>MVTIESDKLRQHDEQLMTKAEQFIIASYRELGKSEQEIKRRVNEIRWEVEQTGTYRHTYEELSYGAKMAWRHSNRCIGRLFWQSLHVIDAREAVTEEEVFSYLFHHIEVATNGGKIRPTITIFRPNGEVRIWNHQLIRYAGYETEEGIIGDSSSLTFTRACEQLGWKGEKTPFDVLPLVIQVGGQKPVWTPIPKELVLEVPIEHPEFPWFRDLQLKWYAVPIISDMCLEIGGIRYMAAPFNGWYMGTEIGARNFADDYRYNMLPKVASCMGLDTNSNASLWKDKA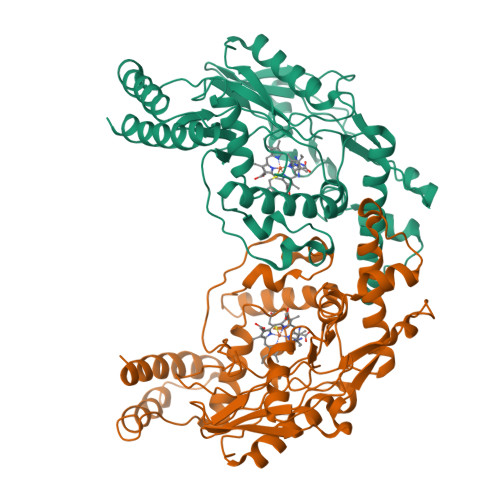LVELNIAVLYSYKKAGVSIVDHHTAARQFQLFEQQEKAAGRHVTGDWTWLIPPLSPATTHIFHRSYDNTMMLPNFFYQDRPYEPQRGEEQ[2x]>[4x]M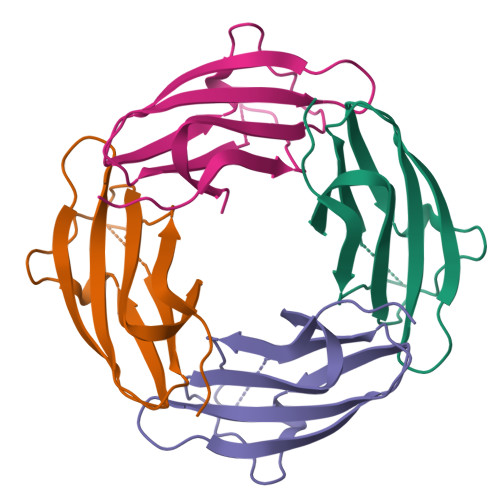SLSIGRTCWAIAEGYIPPYGNGPEPQFISHETVCILNAGDEDAHVEITIYYSDKEPVGPYRLTVPARRTKHVRFNDLNDPAPIPHDTDFASVIQSNVPIVVQHTRLDSRQAENALLSTIAYANTHHHHHH> GPLGSSKMSDVKCTSVVLLSVLQQLRVE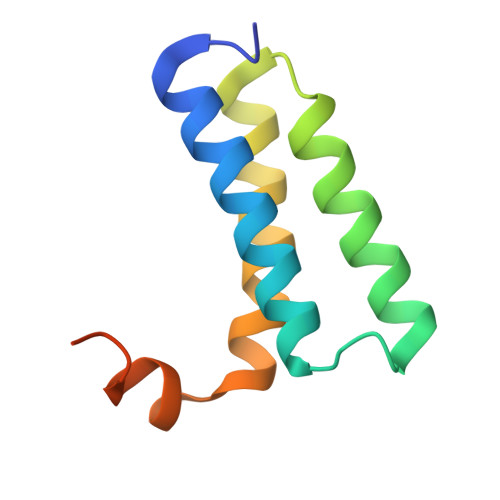SSSKLWAQCVQLHNDILLAKDTTEAFEKMVSLLSVLLSMQGAVDINRLCEEMLDNRATLQ>MGCTLSAEDKAAVERSKMIDRNLREDGERSARLVKILLLGAGESGKSTFLKQMRIIHGQDFDQRAREEFRPTIYSNVIKGMRVLVDAREKLHIPWGDNKNQLHGDKLMAFDTRAPMAAQGMVETRVFLQYLPAIRALWEDSGIQNAYDRRREFQLGESVKYFLDNLDKLGVPDYIPSQQDILLARRPTKGIHEYDFEIKNVPFKMVDVGGQRSERKRWFECFDSVTSILFLVSSSEFDQVLMEDRQTNRLTESLNIFETIVNNRVFSNVSIILFLNKTDLLEEKVQVVSIKDYFLEFEGDPHCLRDVQKFLVECFRGKRRDQQQRPLYHHFTTAINTENIRLVFRDVKDTILHDNLKQLMLQ[2x];>GAMGIQCGGILVPMEDFARGAASPGPSRPGLVPVSIIGAEDEDFENELETNSEEQNSQFQSLEQVKRRPAHLMALLQHVALQFEPGPLLCCLHADMLGSLGPKEAKKAFLDFYHSFLEKTAVLRVPVPPNVAFELDRTRADLISEDVQRRFVQEVVQSQQVAVGRQLEDFRSKRLMGMTPWEQELAQLEAWVGRDRASYEARERHVAERLLMHLEEMQHTISTDEEKSAAV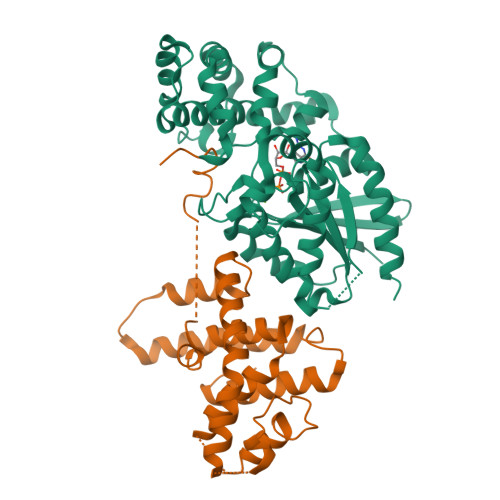VNAIGLYMRHLGVRT[2x]trans-oxyresveratrol | C14 H12 O4 | 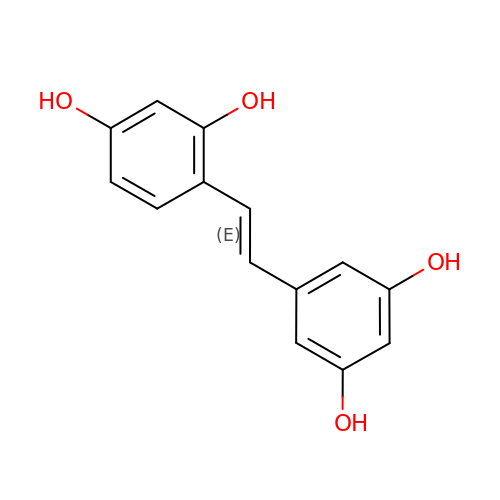PDHAOJSHSJQANO-OWOJBTEDSA-N> MTANNPLYKEAMVALSLKISIGNVVKTMQFEPSTMVYDACRMIRERIPEALAGPPNDFGLFLSDDDPKKGIWLEAGKALDYYMLRNGDTMEYRKKQRPLKI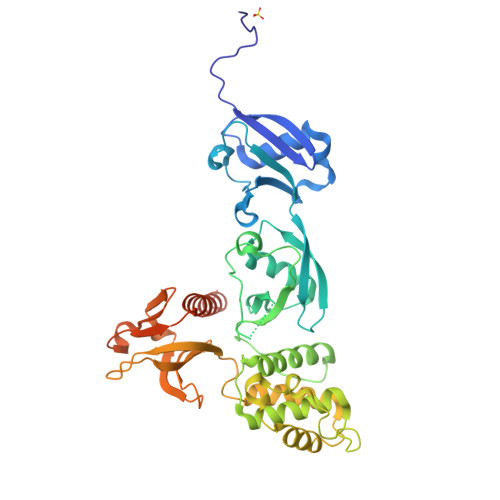RMLDGTVKTIMVDDSKTVTDMLMTICARIGITNHDEYSLVRELMEEKKDELNWLDHGRTLREQGVEEHETLLLRRKFFYSDQNVDSRDPVQLNLLYVQARDDILNGSHPVSFDKACEFAGFQCQIQFGPHNEQKHKAGFLDLKDFLPKEYVKQKGERKIFQAHKNCGQMSEIEAKVRYVKLARSLKTYGVSFFLVKEKMKGKNKLVPRLLGITKECVMRVDEKTKEVIQEWSLTNIKRWAASPKSFTLDFGDYQDGYYSVQTTEGEQIAQLIAGYIRIILKKKKSKDHFGLEGDEESTMLEDSVSPKKST3-(1,3-benzothiazol-2-yl)propanoic acid | C10 H9 N O2 S | 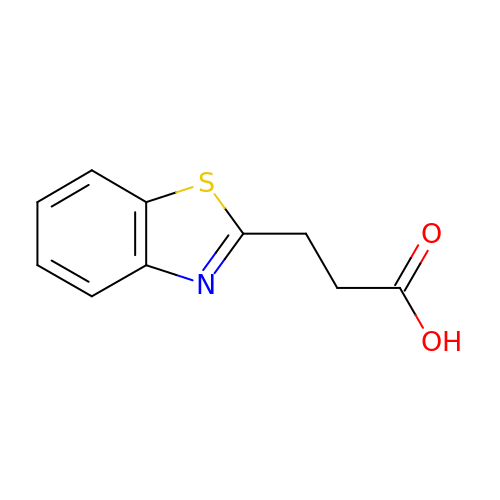WHNQTHDJEZTVHS-UHFFFAOYSA-N> QCTVRYNVADCSHLKLTHIPDDLPSNITVLNLTHNQLRRLPPTNFTRYSQLAILDAGFNSISKLEPELCQILPLLKVLNLQHNELSQISDQTFVFCTNLTELDLMSNSIHKIKSNPFKNQKNLIKLDLS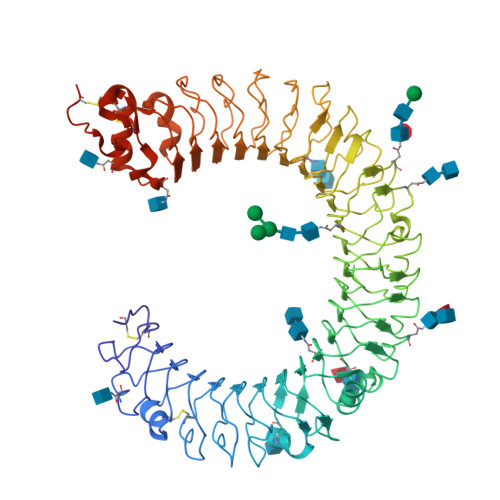HNGLSSTKLGTGVQLENLQELLLAKNKILALRSEELEFLGNSSLRKLDLSSNPLKEFSPGCFQTIGKLFALLLNNAQLNPHLTEKLCWELSNTSIQNLSLANNQLLATSESTFSGLKWTNLTQLDLSYNNLHDVGNGSFSYLPSLRYLSLEYNNIQRLSPRSFYGLSNLRYLSLKRAFTKQSVSLASHPNIDDFSFQWLKYLEYLNMDDNNIPSTKSNTFTGLVSLKYLSLSKTFTSLQTLTNETFVSLAHSPLLTLNLTKNHISKIANGTFSWLGQLRILDLGLNEIEQKLSGQEWRGLRNIFEIYLSYNKYLQLSTSSFALVPSLQRLMLRRVALKNVDISPSPFRPLRNLTILDLSNNNIANINEDLLEGLENLEILDFQHNNLARLWKRANPGGPVNFLKGLSHLHILNLESNGLDEIPVGVFKNLFELKSINLGLNNLNKLEPFIFDDQTSLRSLNLQKNLITSVEKDVFGPPFQNLNSLDMRFNPFDCTCESISWFVNWINQTHTNISELSTHYLCNTPHHYYGFPLKLFDTSSCKDSAPFENLYFQGHHHHHHWSHPQFEK>GVSLRKAERLRAELLDLKAGGFSIRNQKGEQVFRLAFRSGALDLDSCSRDGALLGCSLTADGLPLHFFIQTVRPKDTVMCYRVRWEEAAPGRAVEHAMFLGDAAAHWYGGAEMRTQHWPIRLDGQQEPQPFVTSDVYSSDAAFGGILERYWLSSRAAAIKVNDSVPFHLGWNSTERSLRLQARYHDTPYKPPAGRAAAPELSYRVCVGSDVTSIHKYMVRRYFNKPSRVPAPEAFRDPIWSTWALYGRAVDQDKVLRFAQQIRLHHFNSSHLEIDDMYTPAYGDFDFDEVKFPNASDMFRRLRDAGFRVTLWVHPFVNYNSSRFGEGVERELFVREPTGRLPALVRWWNGIGAVLDFTHPKARDWFQGHLRRLRSRYSVASFKFDAGEVSYLPRDFSTYRPLPDPSVWSRRYTEMALPFFSLAEVRVGYQSQNISCFFRLVNRDSVWGYDLGLRSLIPAVLTVSMLGYPFILPDMVGGNAVPQRTAGGDVPERELYIRWLEVAAFMPAMQFSIPPWRYDAEVVAIAQKFAALRASLVAPLLLELAGEVTDTGDPIVRPLWWIAPGDETAHRIDSQFLIGDTLLVAPVLEPGKQERDVYLPAGKWRSYKGELFDKTPVLLTDYPVDLDEIAYFTWAS[4x]

MYORG is a member of glycoside hydrolase (GH) family 31 (GH31) and, like the other mammalian GH31 enzyme α-glucosidase II, this enzyme is found in the lumen of the endoplasmic reticulum (ER). We were intrigued by MYORG, which is a type II transmembrane protein predicted to be comprised of a short, disordered nucleocytoplasmic N-terminal region, a single transmembrane helix, and a lumenal C-terminal catalytic region comprising a CAZy family glycoside hydrolase 31 (GH31) catalytic domain and 2 β-sheet domains. Here, we demonstrate that MYORG, enigmatically, functions not as an α-glucosidase but rather an α-galactosidase and shows marked preference for specific disaccharide substrates. Recent studies in diverse populations have shown a link between mutations in myogenesis-regulating glycosidase (MYORG) and the development of this disease.

To observe how MYORGGH31 derives its selectivity for Gal-α1,4-Glc, we set out to capture a Michaelis complex with this disaccharide. We used a catalytically impaired variant of MYORG in which the general acid catalytic residue was conservatively mutated (D520N) to allow the intact substrate to bind stably within the active site. After obtaining crystals of this mutant enzyme, we performed ligand soaking experiments. These experiments ultimately yielded structures with unambiguous Fo-Fc electron density for the substrate. Galactose in the −1 subsite is bound in the same position and 4C1 conformation as seen for DGJ, with hydrogen bonding partners being identical other than the endocyclic nitrogen and D520 being swapped for oxygen and N520. Since the wild-type protein binds to DGJ, and the D520N mutant binds to Gal-α1,4-Glc in a near identical manner, we can be confident this is the interaction network the wild-type protein uses to bind Gal-α1,4-Glc during catalysis. The glucose residue bound in the +1 site is held in position through hydrogen bonding interactions to D213 and R504, while stacking interactions between the pyranose ring of the glucose residue and W426 likely serve to increase the overall affinity for Gal-α1,4-Glc towards MYORG. In particular, the binary substrate complex of MYORG bound to Gal-α1,4-Glc explains both its requirement for galactosides binding within the −1 subsite and strong preference for glucose binding within the +1 binding site. In summary, the shape of the +1 subsite dictates specificity for α1,4-Glc since alternative linkages and monosaccharides bound in this site would form unproductive steric clashes. To assess the catalytic proficiency of MYORG on this disaccharide, we performed more detailed kinetic analysis and were able to observe Michaelis–Menten kinetics that yielded values for KM (980 ± 7 μM), kcat (0.047 ± 0.003 min−1), and kcat/KM (49 ± 7 M−1 min−1).> MSFESKKPMRTWSHLAEMRKKPSEYDIVSRKLHYSTNNPDSPWELSPDSPMNLWYKQYRNASPLKHDNWDAFTDPDQLVYRTYNLMQDGQESYVQSLFDQFNEREHDQMVREGWEHTMARCYSPLRYLFHCLQMSSAYVQQMAPASTISNCCILQTADSLRWLTHTAY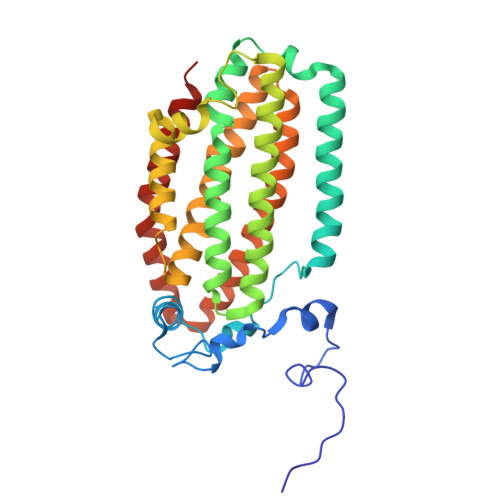RTHELSLTYPDAGLGEHERELWEKEPGWQGLRELMEKQLTAFDWGEAFVSLNLVVKPMIVESIFKPLQQQAWENNDTLLPLLIDSQLKDAERHSRWSKALVKHALENPDNHAVIEGWIEKWRPLADRAAEAYLSMLSSD>PENITFDTLNTQNDHEETYGESPEVPKASIAPAGRQNVPVLQQNQENEDNHALGGSEDAKDEREIQSSAIKTLYNYYSEGPSTPIMPHLVNRLRGLDALAKVDATLSKVDMNAAYIFALRPTFPYSYGYKQRFSNRRLTTSALCYARTGLSSFLTVDKTYTSNSPLKGGSRGWPIFNVGVSPHVAEPHMRTLSPIGLEVFNLATSQFSKTLLTASSKVFTQSLYTADILSI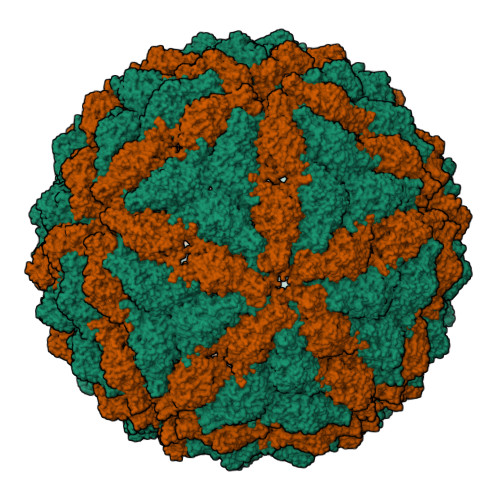FGEVFLPHVMQPVSNYTPILVRALLALIHILGSGSGNCSLSSSIFESSIPQFLTISHSTNMSNRTRYCLHTWSAYKDMFRNGIPPQSTFPPTLAPEGSSARILIPAALVTSPMFPWLLVLVSSGPQFFLYSKDASINTVDIGSRGRITSPIPDVAHLDLHRLWNLFRFDGYRYIDVVIVGVDRDYVWPYQNGVYVHGGKGPKGTDNYENADVHDGIGTIFSSFNNNVNVQTSDLLLGLSTLWNHITTTYATEEEVTMAIKIAAAFALVYPVQPIVYSGCSRALYNHTSYFQPSSENCYTTDTAEVKSTWDTVELSVQVNNAMVLGMTLPFGQPTVSSAQWFNNIDKAEISMFKVGNLPLQNLDYLSLDMMEFYAPTTGQLYDIRSDSLISSAHRTVNLGIGYTALADFFAYLASVPAQSFYHNRMVTSPISKQAYSVYERFIERFIDDFVGWGRCDLFNLDTLLGAKRIAGVASSPIPWHCSLQRCPLPIIMHYTGLHFGQEHIRVRDVAGVEGLQQIVLRNDQGSIVLDALGTAAPSRLAVKLDWSRLSAWYSDTTCAIPISDRVMEIVNYAAIWDPTQERRATGFVYTYFSPNFLSSFNVSEPIFNKTINLTPPYDDTSQTVIQNLSMPQMLSFDPYYESTFYVVSADNEWVPTSGPAWKVPYLENVVKRSGRRLLAELRIASNNGSGDRTFLDDV[2x]> QQLPQPSLSLHPSQGVSLGDTVTLRCHLPRMAAWVQLWLNGTLRFDKEKDKEQDAAEFSFAVTNLEDAGTYQCRYQVSEPLWTSNQSDPVELVL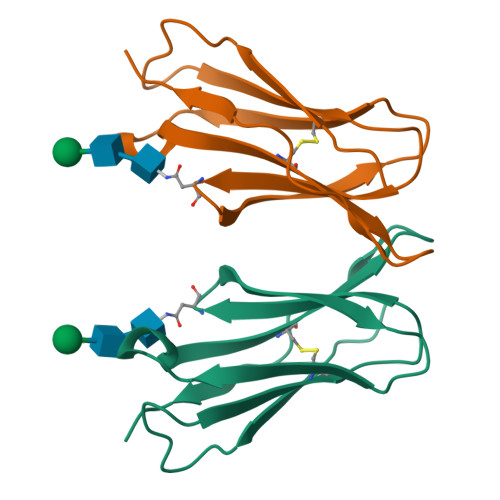TIEGRHHHHHH>MQGVNIYNISAGTSVDLAAPVTTGDIVTFFSSALN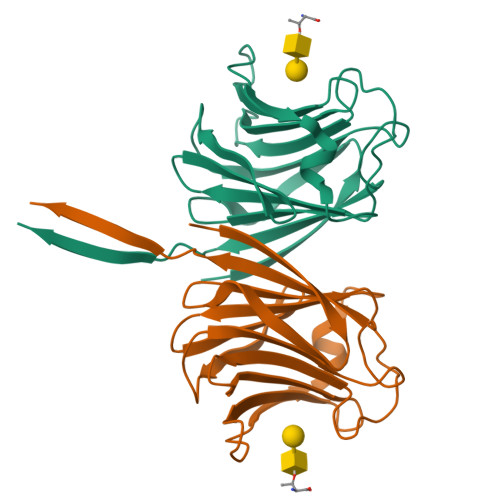LNAGAGNPNNTTLNLFAENGAYLLHIAFRLQENVIIFNSRQPDGPWLVEQRVSDVANQFAGIDGKAMVTVFDHGDKYQVVINEKTVIQYTKQISGLTSSLSYNATEETSIFSTVVEAVTYTGLALEHHHHHH[2x]> MADVINVSVNLEAFSQAISAIQALRSSVSRVFDCLKDGMRNKETLEGREKAFIAHFQDNLHSVNRDLNELERLSNLVGKPSENHPLHNSGLLSLDPVQDKTPLYSQLLQAYKWSNKLQYHAGLASGLLNQQSLKRSANQMGVSAKRRPKAQPTTLVLPPQYVDDVISRIDRMFPEMSIHLSRPNGTSAMLLVTLGKVLKVIVVMRSLFIDRTIVKGYNENVYTEDGKLDIWSKSNYQVFQKVTDHATTALLHYQLPQMPDVVVRSFMTWLRSYIKLFQAPCQRCGKFLQDGLPPTWRDFRTLEAFHDTCRQ;> MAAPLGGMFSGQPPGPPQAPPGLPGQASLLQAAPGAPRPSSSTLVDELESSFEACFASLVSQDYVNGTDQEEIRTGVDQCIQKFLDIARQTECFFLQKRLQLSVQKPEQVIKEDVSELRNELQRKDALVQKHLTKLRHWQQVLEDINVQHKKPADIPQGSLAYLEQASANIPAPLKPT;> MAASQQQASAASSAAGVSGPSSAGGPGPQQQPQPPAQLVGPAQSGLLQQQQQDFDPVQRYKMLIPQLKESLQTLMKVAAQNLIQNTNIDNGQKSSDGPIQRFDKCLEEFYALCDQLELCLRLAHECLSQSCDSAKHSPTLVPTATKPDAVQPDSLPYPQYLAVIKAQISCAKDIHTALLDCANKVTGKTPAPPAGPGGTL;> MSTPPLAASGMAPGPFAGPQAQQAAREVNTASLCRIGQETVQDIVYRTMEIFQLLRNMQLPNGVTYHTGTYQDRLTKLQDNLRQLSVLFRKLRLVYDKCNENCGGMDPIPVEQLIPYVEEDGSKNDDRAGPPRFASEERREIAEVNKKLKQKNQQLKQIMDQLRNLIWDINAMLAMRN;> MAAAVAMETDDAGNRLRFQLELEFVQCLANPNYLNFLAQRGYFKDKAFVNYLKYLLYWKDPEYAKYLKYPQCLHMLELLQYEHFRKELVNAQCAKFIDEQQILHWQHYSRKRMRLQQALAEQQQQNNTSGK;> MKAQGETEESEKLSKMSSLLERLHAKFNQNRPWSETIKLVRQVMEKRVVMSSGGHQHLVSCLETLQKALKVTSLPAMTDRLESIARQNGLGSHLSASGTECYITSDMFYVEVQLDPAGQLCDVKVAHHGENPVSCPELVQQLREKNFDEFSKHLKGLVNLYNLPGDNKLKTKMYLALQSLEQDLSKMAIMYWKATNAGPLDKILHGSVGYLTPRSGGHLMNLKYYVSPSDLLDDKTASPIILHENNVSRSLGMNASVTIEGTSAVYKLPIAPLIMGSHPVDNKWTPSFSSITSANSVDLPACFFLKFPQPIPVSRAFVQKLQNCTGIPLFETQPTYAPLYELITQFELSKDPDPIPLNHNM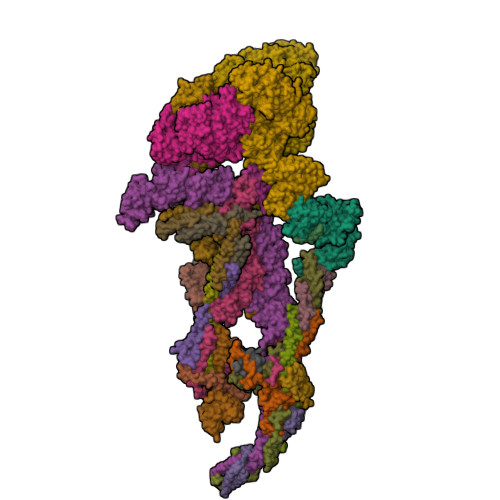RFYAALPGQQHCYFLNKDAPLPDGRSLQGTLVSKITFQHPGRVPLILNLIRHQVAYNTLIGSCVKRTILKEDSPGLLQFEVCPLSESRFSVSFQHPVNDSLVCVVMDVQDSTHVSCKLYKGLSDALICTDDFIAKVVQRCMSIPVTMRAIRRKAETIQADTPALSLIAETVEDMVKKNLPPASSPGYGMTTGNNPMSGTTTPTNTFPGGPITTLFNMSMSIKDRHESVGHGEDFSKVSQNPILTSLLQITGNGGSTIGSSPTPPHHTPPPVSSMAGNTKNHPMLMNLLKDNPAQDFSTLYGSSPLERQNSSSGSPRMEICSGSNKTKKKKSSRLPPEKPKHQTEDDFQRELFSMDVDSQNPIFDVNMTADTLDTPHITPAPSQCSTPPTTYPQPVPHPQPSIQRMVRLSSSDSIGPDVTDILSDIAEEASKLPSTSDDCPAIGTPLRDSSSSGHSQSTLFDSDVFQTNNNENPYTDPADLIADAAGSPSSDSPTNHFFHDGVDFNPDLLNSQSQSGFGEEYFDESSQSGDNDDFKGFASQALNTLGVPMLGGDNGETKFKGNNQADTVDFSIISVAGKALAPADLMEHHSGSQGPLLTTGDLGKEKTQKRVKEGNGTSNSTLSGPGLDSKPGKRSRTPSNDGKSKDKPPKRKKADTEGKSPSHSSSNRPFTPPTSTGGSKSPGSAGRSQTPPGVATPPIPKITIQIPKGTVMVGKPSSHSQYTSSGSVSSSGSKSHHSHSSSSSSSASTSGKMKSSKSEGSSSSKLSSSMYSSQGSSGSSQSKNSSQSGGKPGSSPITKHGLSSGSSSTKMKPQGKPSSLMNPSLSKPNISPSHSRPPGGSDKLASPMKPVPGTPPSSKAKSPISSGSGGSHMSGTSSSSGMKSSSGLGSSGSLSQKTPPSSNSCTASSSSFSSSGSSMSSSQNQHGSSKGKSPSRNKKPSLTAVIDKLKHGVVTSGPGGEDPLDGQMGVSTNSSSHPMSSKHNMSGGEFQGKREKSDKDKSKVSTSGSSVDSSKKTSESKNVGSTGVAKIIISKHDGGSPSIKAKVTLQKPGESSGEGLRPQMASSKNYGSPLISGSTPKHERGSPSHSKSPAYTPQNLDSESESGSSIAEKSYQNSPSSDDGIRPLPEYSTEKHKKHKKEKKKVKDKDRDRDRDKDRDKKKSHSIKPESWSKSPISSDQSLSMTSNTILSADRPSRLSPDFMIGEEDDDLMDVALIGN;> AAAAAAAAAAAAAAAAAAAA;> MAASSSGEKEKERLGGGLGVAGGNSTRERLLSALEDLEVLSRELIEMLAISRNQKLLQAGEENQVLELLIHRDGEFQELMKLALNQGKIHHEMQVLEKEVEKRDSDIQQLQKQLKEAEQILATAVYQAKEKLKSIEKARKGAISSEEIIKYAHRISASNAVCAPLTWVPGDPRRPYPTDLEMRSGLLGQMNNPSTNGVNGHLPGDALAAGRLPDVLAPQYPWQSNDMSMNMLPPNHSSDFLLEPPGHNKENEDDVEIMSTDSSSSSSESD;> MAAVDIRDNLLGISWVDSSWIPILNSGSVLDYFSERSNPFYDRTCNNEVVKMQRLTLEHLNQMVGIEYILLHAQEPILFIIRKQQRQSPAQVIPLADYYIIAGVIYQAPDLGSVINSRVLTAVHGIQSAFDEAMSYCRYHPSKGYWWHFKDHEEQDKVRPKAKRKEEPSSIFQRQRVDALLLDLRQKFPPKFVQLKPGEKPVPVDQTKKEAEPIPETVKPEEKETTKNVQQTVSAKGPPEKRMRLQ;> MGEPQQVSALPPPPMQYIKEYTDENIQEGLAPKPPPPIKDSYMMFGNQFQCDDLIIRPLESQGIERLHPMQFDHKKELRKLNMSILINFLDLLDILIRSPGSIKREEKLEDLKLLFVHVHHLINEYRPHQARETLRVMMEVQKRQRLETAERFQKHLERVIEMIQNCLASLPDDLPHSEAGMRVKTEPMDADDSNNCTGQNEHQRENSGHRRDQIIEKDAALCVLIDEMNERP;> MQREEKQLEASLDALLSQVADLKNSLGSFICKLENEYGRLTWPSVLDSFALLSGQLNTLNKVLKHEKTPLFRNQVIIPLVLSPDRDEDLMRQTEGRVPVFSHEVVPDHLRTKPDPEVEEQEKQLTTDAARIGADAAQKQIQSLNKMCSNLLEKISKEERESESGGLRPNKQTFNPTDTNALVAAVAFGKGLSNWRPSGSSGPGQAGQPGAGTILAGTSGLQQVQMAGAPSQQQPMLSGVQMAQAGQPGKMPSGIKTNIKSASMHPYQR;> MASAGVAAGRQAEDVLPPTSDQPLPDTKPLPPPQPPPVPAPQPQQSPAPRPQSPARAREEENYSFLPLVHNIIKCMDKDSPEVHQDLNALKSKFQEMRKLISTMPGIHLSPEQQQQQLQSLREQVRTKNELLQKYKSLCMFEIPKE;> MAEKFDHLEEHLEKFVENIRQLGIIVSDFQPSSQAGLNQKLNFIVTGLQDIDKCRQQLHDITVPLEVFEYIDQGRNPQLYTKECLERALAKNEQVKGKIDTMKKFKSLLIQELSKVFPEDMAKYRSIRGEDHPPS;> MATYSLANERLRALEDIEREIGAILQNAGTVILELSKEKTNERLLDRQAAAFTASVQHVEAELSAQIRYLTQVATGQPHEGSSYSSRKDCQMALKRVDYARLKLSDVARTCEQMLEN;> MAPVQLENHQLVPPGGGGGGSGGPPSAPAPPPPGAAVAAAAAAAASPGYRLSTLIEFLLHRAYSELMVLTDLLPRKSDVERKIEIVQFASRTRQLFVRLLALVKWANNAGKVEKCAMISSFLDQQAILFVDTADRLASLARDALVHARLPSFAIPYAIDVLTTGSYPRLPTCIRDKIIPPDPITKIEKQATLHQLNQILRHRLVTTDLPPQLANLTVANGRVKFRVEGEFEATLTVMGDDPDVPWRLLKLEILVEDKETGDGRALVHSMQISFIHQLVQSRLFADEKPLQDMYNCLHSFCLSLQLEVLHSQTLMLIRERWGDLVQVERYHAGKCLSLSVWNQQVLGRKTGTASVHKVTIKIDENDVSKPLQIFHDPPLPASDSKLVERAMKIDHLSIEKLLIDSVHARAHQKLQELKAILRGFNANENSSIETALPALVVPILEPCGNSECLHIFVDLHSGMFQLMLYGLDQATLDDMEKSVNDDMKRIIPWIQQLKFWLGQQRCKQSIKHLPTISSETLQLSNYSTHPIGNLSKNKLFIKLTRLPQYYIVVEMLEVPNKPTQLSYKYYFMSVNAADREDSPAMALLLQQFKENIQDLVFRTKTGKQTRTNAKRKLSDDPCPVESKKTKRAGEMCAFNKVLAHFVAMCDTNMPFVGLRLELSNLEIPHQGVQVEGDGFSHAIRLLKIPPCKGITEETQKALDRSLLDCTFRLQGRNNRTWVAELVFANCPLNGTSTREQGPSRHVYLTYENLLSEPVGGRKVVEMFLNDWNSIARLYECVLEFARSLPDIPAHLNIFSEVRVYNYRKLILCYGTTKGSSISIQWNSIHQKFHISLGTVGPNSGCSNCHNTILHQLQEMFNKTPNVVQLLQVLFDTQAPLNAINKLPTVPMLGLTQRTNTAYQCFSILPQSSTHIRLAFRNMYCIDIYCRSRGVVAIRDGAYSLFDNSKLVEGFYPAPGLKTFLNMFVDSNQDARRRSVNEDDNPPSPIGGDMMDSLISQLQPPPQQQPFPKQPGTSGAYPLTSPPTSYHSTVNQSPSMMHTQSPGNLHAASSPSGALRAPSPASFVPTPPPSSHGISIGPGASFASPHGTLDPSSPYTMVSPSGRAGNWPGSPQVSGPSPAARMPGMSPANPSLHSPVPDASHSPRAGTSSQTMPTNMPPPRKLPQRSWAASIPTILTHSALNILLLPSPTPGLVPGLAGSYLCSPLERFLGSVIMRRHLQRIIQQETLQLINSNEPGVIMFKTDALKCRVALSPKTNQTLQLKVTPENAGQWKPDELQVLEKFFETRVAGPPFKANTLIAFTKLLGAPTHILRDCVHIMKLELFPDQATQLKWNVQFCLTIPPSAPPIAPPGTPAVVLKSKMLFFLQLTQKTSVPPQEPVSIIVPIIYDMASGTTQQADIPRQQNSSVAAPMMVSNILKRFAEMNPPRQGECTIFAAVRDLMANLTLPPGGRP;> MDVSGQETDWRSTAFRQKLVSQIEDAMRKAGVAHSKSSKDMESHVFLKAKTRDEYLSLVARLIIHFRDIHNKKSQASVSDPMNALQSLTGGPAAGAAGIGMPPRGPGQSLGGMGSLGAMGQPMSLSGQPPPGTSGMAPHSMAVVSTATPQTQLQLQQVALQQQQQQQQFQQQQQAALQQQQQQQQQQQFQAQQSAMQQQFQAVVQQQQQLQQQQQQQQHLIKLHHQNQQQIQQQQQQLQRIAQLQLQQQQQQQQQQQQQQQQALQAQPPIQQPPMQQPQPPPSQALPQQLQQMHHTQHHQPPPQPQQPPVAQNQPSQLPPQSQTQPLVSQAQALPGQMLYTQPPLKFVRAPMVVQQPPVQPQVQQQQTAVQTAQAAQMVAPGVQMITEALAQGGMHIRARFPPTTAVSAIPSSSIPLGRQPMAQVSQSSLPMLSSPSPGQQVQTPQSMPPPPQPSPQPGQPSSQPNSNVSSGPAPSPSSFLPSPSPQPSQSPVTARTPQNFSVPSPGPLNTPVNPSSVMSPAGSSQAEEQQYLDKLKQLSKYIEPLRRMINKIDKNEDRKKDLSKMKSLLDILTDPSKRCPLKTLQKCEIALEKLKNDMAVPTPPPPPVPPTKQQYLCQPLLDAVLANIRSPVFNHSLYRTFVPAMTAIHGPPITAPVVCTRKRRLEDDERQSIPSVLQGEVARLDPKFLVNLDPSHCSNNGTVHLICKLDDKDLPSVPPLELSVPADYPAQSPLWIDRQWQYDANPFLQSVHRCMTSRLLQLPDKHSVTALLNTWAQSVHQACLSAA;> MCDLRRPAAGGMMDLAYVCEWEKWSKSTHCPSVPLACAWSCRNLIAFTMDLRSDDQDLTRMIHILDTEHPWDLHSIPSEHHEAITCLEWDQSGSRLLSADADGQIKCWSMADHLANSWESSVGSLVEGDPIVALSWLHNGVKLALHVEKSGASSFGEKFSRVKFSPSLTLFGGKPMEGWIAVTVSGLVTVSLLKPSGQVLTSTESLCRLRGRVALADIAFTGGGNIVVATADGSSASPVQFYKVCVSVVSEKCRIDTEILPSLFMRCTTDLNRKDKFPAITHLKFLARDMSEQVLLCASSQTSSIVECWSLRKEGLPVNNIFQQISPVVGDKQPTILKWRILSATNDLDRVSAVALPKLPISLTNTDLKVASDTQFYPGLGLALAFHDGSVHIVHRLSLQTMAVFYSSAAPRPVDEPAMKRPRTAGPAVHLKAMQLSWTSLALVGIDSHGKLSVLRLSPSMGHPLEVGLALRHLLFLLEYCMVTGYDWWDILLHVQPSMVQSLVEKLHEEYTRQTAALQQVLSTRILAMKASLCKLSPCTVTRVCDYHTKLFLIAISSTLKSLLRPHFLNTPDKSPGDRLTEICTKITDVDIDKVMINLKTEEFVLDMNTLQALQQLLQWVGDFVLYLLASLPNQGSLLRPGHSFLRDGTSLGMLRELMVVIRIWGLLKPSCLPVYTATSDTQDSMSLLFRLLTKLWICCRDEGPASEPDEALVDECCLLPSQLLIPSLDWLPASDGLVSRLQPKQPLRLQFGRAPTLPGSAATLQLDGLARAPGQPKIDHLRRLHLGACPTEECKACTRCGCVTMLKSPNRTTAVKQWEQRWIKNCLCGGLWWRVPLSYP;> MSGVRAVRISIESACEKQVHEVGLDGTETYLPPLSMSQNLARLAQRIDFSQGSGSEEEEAAGTEGDAQEWPGAGSSADQDDEEGVVKFQPSLWPWDSVRNNLRSALTEMCVLYDVLSIVRDKKFMTLDPVSQDALPPKQNPQTLQLISKKKSLAGAAQILLKGAERLTKSVTENQENKLQRDFNSELLRLRQHWKLRKVGDKILGDLSYRSAGSLFPHHGTFEVIKNTDLDLDKKIPEDYCPLDVQIPSDLEGSAYIKVSIQKQAPDIGDLGTVNLFKRPLPKSKPGSPHWQTKLEAAQNVLLCKEIFAQLSREAVQIKSQVPHIVVKNQIISQPFPSLQLSISLCHSSNDKKSQKFATEKQCPEDHLYVLEHNLHLLIREFHKQTLSSIMMPHPASAPFGHKRMRLSGPQAFDKNEINSLQSSEGLLEKIIKQAKHIFLRSRAAATIDSLASRIEDPQIQAHWSNINDVYESSVKVLITSQGYEQICKSIQLQLNIGVEQIRVVHRDGRVITLSYQEQELQDFLLSQMSQHQVHAVQQLAKVMGWQVLSFSNHVGLGPIESIGNASAITVASPSGDYAISVRNGPESGSKIMVQFPRNQCKDLPKSDVLQDNKWSHLRGPFKEVQWNKMEGRNFVYKMELLMSALSPCLL;> MEAPPVTMMPVTGGTINMMEYLLQGSVLDHSLESLIHRLRGLCDNMEPETFLDHEMVFLLKGQQASPFVLRARRSMDRAGAPWHLRYLGQPEMGDKNRHALVRNCVDIATSENLTDFLMEMGFRMDHEFVAKGHLFRKGIMKIMVYKIFRILVPGNTDSTEALSLSYLVELSVVAPAGQDMVSDDMKNFAEQLKPLVHLEKIDPKRLM;> MENFTALFGAQADPPPPPTALGFGPGKPPPPPPPPAGGGPGTAPPPTAATAPPGADKSGAGCGPFYLMRELPGSTELTGSTNLITHYNLEQAYNKFCGKKVKEKLSNFLPDLPGMIDLPGSHDNSSLRSLIEKPPILSSSFNPITGTMLAGFRLHTGPLPEQCRLMHIQPPKKKNKHKHKQSRTQDPVPPETPSDSDHKKKKKKKEEDPDRKRKKKEKKKKKNRHSPDHPGMGSSQASSSSSLR;> MGVTCVSQMPVAEGKSVQQTVELLTRKLEMLGAEKQGTFCVDCETYHTAASTLGSQGQTGKLMYVMHNSEYPLSCFALFENGPCLIADTNFDVLMVKLKGFFQSAKASKIETRGTRYQYCDFLVKVGTVTMGPSARGISVEVEYGPCVVASDCWSLLLEFLQSFLGSHTPGAPAVFGNRHDAVYGPADTMVQYMELFNKIRKQQQVPVAGIR;> MADRLTQLQDAVNSLADQFCNAIGVLQQCGPPASFNNIQTAINKDQPANPTEEYAQLFAALIARTAKDIDVLIDSLPSEESTAALQAASLYKLEEENHEAATCLEDVVYRGDMLLEKIQSALADIAQSQLKTRSGTHSQSLPDS;> MAQQRALPQSKETLLQSYNKRLKDDIKSIMDNFTEIIKTAKIEDETQVSRATQGEQDNYEMHVRAANIVRAGESLMKLVSDLKQFLILNDFPSVNEAIDQRNQQLRTLQEECDRKLITLRDEISIDLYELEEEYYSSSSSLCEANDLPLCEAYGRLDLDTDSADGLSAPLLASPEPSAGPLQVAAPAHSHAGGPGPTEHA;> METQLQSIFEEVVKTEVIEEAFPGMFMDTPEDEKTKLISCLGAFRQFWGGLSQESHEQCIQWIVKFIHGQHSPKRISFLYDCLAMAVETGLLPPRLVCESLINSDTLEWERTQLWALTFKLVRKIIGGVDYKGVRDLLKVILEKILTIPNTVSSAVVQQLLAAREVIAYILERNACLLPAYFAVTEIRKLYPEGKLPHWLLGNLVSDFVDTFRPTARINSICGRCSLLPVVNNSGAICNSWKLDPATLRFPLKGLLPYDKDLFEPQTALLRYVLEQPYSRDMVCNMLGLNKQHKQRCPVLEDQLVDLVVYAMERSETEEKFDDGGTSQLLWQHLSSQLIFFVLFQFASFPHMVLSLHQKLAGRGLIKGRDHLMWVLLQFISGSIQKNALADFLPVMKLFDLLYPEKEYIPVPDINKPQSTHAFAMTCIWIHLNRKAQNDNSKLQIPIPHSLRLHHEFLQQSLRNKSLQMNDYKIALLCNAYSTNSECFTLPMGALVETIYGNGIMRIPLPGTNCMASGSITPLPMNLLDSLTVHAKMSLIHSIATRVIKLAHAKSSVALAPALVETYSRLLVYMEIESLGIKGFISQLLPTVFKSHAWGILHTLLEMFSYRMHHIQPHYRVQLLSHLHTLAAVAQTNQNQLHLCVESTALRLITALGSSEVQPQFTRFLSDPKTVLSAESEELNRALILTLARATHVTDFFTGSDSIQGTWCKDILQTIMSFTPHNWASHTLSCFPGPLQAFFKQNNVPQESRFNLKKNVEEEYRKWKSMSNENDIITHFSMQGSPPLFLCLLWKMLLETDHINQIGYRVLERIGARALVAHVRTFADFLVYEFSTSAGGQQLNKCIEILNDMVWKYNIVTLDRLILCLAMRSHEGNEAQVCYFIIQLLLLKPNDFRNRVSDFVKENSPEHWLQNDWHTKHMNYHKKYPEKLYFEGLAEQVDPPVQIQSPYLPIYFGNVCLRFLPVFDIVIHRFLELLPVSKSLETLLDHLGGLYKFHDRPVTYLYNTLHYYEMHLRDRAFLKRKLVHAIIGSLKDNRPQGWCLSDTYLKCAMNAREENPWVPDDTYYCRLIGRLVDTMAGKSPGPFPNCDWRFNEFPNPAAHALHVTCVELMALAVSGKEVGNALLNVVLKSQPLVPRENITAWMNAIGLIITALPEPYWIVLHDRIVSVISSPSLTSETEWVGYPFRLFDFTACHQSYSEMSCSYTLALAHAVWHHSSIGQLSLIPKFLTEVLLPIVKTEFQLLYVYHLVGPFLQRFQQERTRCMIEIGVAFYDMLLNVDQCSTHLNYMDPICDFLYHMKYMFTGDSVKEQVEKIICNLKPALKLRLRFITHISKMEPAAVPPQAMNSGSPAPQSNQVPVSLPVTQ;> MKVVNLKQAILQAWKERWSDYQWAINMKKFFPKGATWDILNLADALLEQAMIGPSPNPLILSYLKYAISSQMVSYSSVLTAISKFDDFSRDLCVQALLDIMDMFCDRLSCHGKAEECIGLCRALLSALHWLLRCTAASAERLREGLEAGTPAAGEKQLAMCLQRLEKTLSSTKNRALLHIAKLEEASSWTAIEHSLLKLGEILANLSNPQLRSQAEQCGTLIRSIPTMLSVHAEQMHKTGFPTVHAVILLEGTMNLTGETQSLVEQLTMVKRMQHIPTPLFVLEIWKACFVGLIESPEGTEELKWTAFTFLKIPQVLVKLKKYSHGDKDFTEDVNCAFEFLLKLTPLLDKADQRCNCDCTNFLLQECGKQGLLSEASVNNLMAKRKADREHAPQQKSGENANIQPNIQLILRAEPTVTNILKTMDADHSKSPEGLLGVLGHMLSGKSLDLLLAAAAATGKLKSFARKFINLNEFTTYGSEESTKPASVRALLFDISFLMLCHVAQTYGSEVILSESRTGAEVPFFETWMQTCMPEEGKILNPDHPCFRPDSTKVESLVALLNNSSEMKLVQMKWHEACLSISAAILEILNAWENGVLAFESIQKITDNIKGKVCSLAVCAVAWLVAHVRMLGLDEREKSLQMIRQLAGPLFSENTLQFYNERVVIMNSILERMCADVLQQTATQIKFPSTGVDTMPYWNLLPPKRPIKEVLTDIFAKVLEKGWVDSRSIHIFDTLLHMGGVYWFCNNLIKELLKETRKEHTLRAVELLYSIFCLDMQQVTLVLLGHILPGLLTDSSKWHSLMDPPGTALAKLAVWCALSSYSSHKGQASTRQKKRHREDIEDYISLFPLDDVQPSKLMRLLSSNEDDANILSSPTDRSMSSSLSASQLHTVNMRDPLNRVLANLFLLISSILGSRTAGPHTQFVQWFMEECVDCLEQGGRGSVLQFMPFTTVSELVKVSAMSSPKVVLAITDLSLPLGRQVAAKAIAAL;> MVPGSEGPARAGSVVADVVFVIEGTANLGPYFEGLRKHYLLPAIEYFNGGPPAETDFGGDYGGTQYSLVVFNTVDCAPESYVQCHAPTSSAYEFVTWLDGIKFMGGGGESCSLIAEGLSTALQLFDDFKKMREQIGQTHRVCLLICNSPPYLLPAVESTTYSGCTTENLVQQIGERGIHFSIVSPRKLPALRLLFEKAAPPALLEPLQPPTDVSQDPRHMVLVRGLVLPVGGGSAPGPLQSKQPVPLPPAAPSGATLSAAPQQPLPPVPPQYQVPGNLSAAQVAAQNAVEAAKNQKAGLGPRFSPITPLQQAAPGVGPPFSQAPAPQLPPGPPGAPKPPPASQPSLVSTVAPGSGLAPTAQPGAPSMAGTVAPGGVSGPSPAQLGAPALGGQQSVSNKLLAWSGVLEWQEKPKPASVDANTKLTRSLPCQVYVNHGENLKTEQWPQKLIMQLIPQQLLTTLGPLFRNSRMVQFHFTNKDLESLKGLYRIMGNGFAGCVHFPHTAPCEVRVLMLLYSSKKKIFMGLIPYDQSGFVNGIRQVITNHKQVQQQKLEQQQRGMGGQQAPPGLGPILEDQARPSQNLLQLRPPQPQPQGTVGASGATGQPQPQGTAQPPPGAPQGPPGAASGPPPPGPILRPQNPGANPQLRSLLLNPPPPQTGVPPPQASLHHLQPPGAPALLPPPHQGLGQPQLGPPLLHPPPAQSWPAQLPPRAPLPGQMLLSGGPRGPVPQPGLQPSVMEDDILMDLI;> MTAAPASPQQIRDRLLQAIDPQSNIRNMVAVLEVISSLEKYPITKEALEETRLGKLINDVRKKTKNEELAKRAKKLLRSWQKLIEPAHQHEAALRGLAGATGSANGGAHNCRPEVGAAGPPRSIHDLKSRNDLQRLPGQRLDRLGSRKRRGDQRDLGHPGPPPKVSKASHDPLVPNSSPLPTNGISGSPESFASSLDGSGHAGPEGSRLERDENDKHSGKIPVNAVRPHTSSPGLGKPPGPCLQPKASVLQQLDRVDETPGPPHPKGPPRCSFSPRNSRHEGSFARQQSLYAPKGSVPSPSPRPQALDATQVPSPLPLAQPSTPPVRRLELLPSAESPVCWLEQPESHQRLAGPGCKAGLSPAEPLLSRAGFSPDSSKADSDAASSGGSDSKKKKRYRPRDYTVNLDGQVAEAGVKPVRLKERKLTFDPMTRQIKPLTQKEPVRADSPVHMEQQSRTELDKQEAKASLQSPFEQTNWKELSRNEIIQSYLSRQSSLLSSSGAQTPGAHHFMSEYLKQEESTRQGARQLHVLVPQSPPTDLPGLTREVTQDDLDRIQASQWPGVNGCQDTQGNWYDWTQCISLDPHGDDGRLNILPYVCLD>NHHHHHHPCCSNPCQNRGECMSTGFDQYKCDCTRTGFYGENCTTPEFLTRIKLLLKPTPNTVHYILTHFKGVWNIVNNIPFLRSLIMKYVLTSRSYLIDSPPTYNVHYGYKSWEAFSNLSYYTRALPPVADDCPTPMGVKGNKELPDSKEVLEKVLLRREFIPDPQGSNMMFAFFAQHFTHQFFKTDHKRGPGFTRGLGHGVDLNHIYGETLDRQHKLRLFKDGKLKYQVIGGEVYPPTVKDTQVEMIYPPHIPENLQFAVGQEVFGLVPGLMMYATIWLREHNRVCDILKQEHPEWGDEQLFQTSRLILIGETIKIVIEDYVQHLSGYHFKLKFDPELLFNQQFQYQNRIASEFNTLYHWHPLLPDTFNIEDQEYSFKQFLYNNSILLEHGLTQFVESFTRQIAGRVAGGRNVPIAVQAVAKASIDQSREMKYQSLNEYRKRFSLKPYTSFEELTGEKEMAAELKALYSDIDVMELYPALLVEKP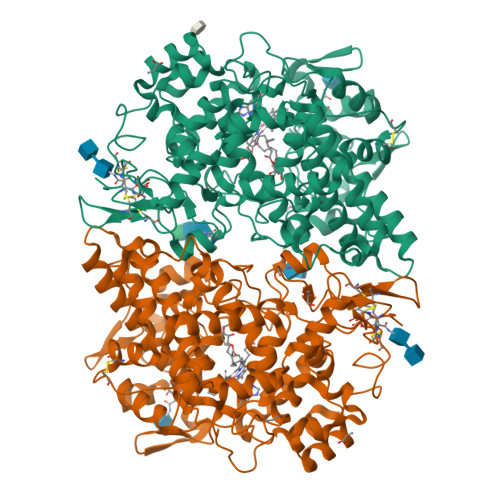RPDAIFGETMVELGAPFSLKGLMGNPICSPQYWKPSTFGGEVGFKIINTASIQSLICNNVKGCPFTSFNVQDPQPTKTATIAASASHSRLDDINPTVLIKR[2x]>GHMGEVLTVFHAGSLSVPFEELEAEFEAQHPGVDVQREAAGSAQSVRKITELGKKADVLASADYALIPSLMVPEYADWYAAFARNQMILAYTNESKYGDEINTDNWYEILRRPDVRYGFSNPNDDPAGYRSQMVTQLAESYYNDDMIYDDLMLANTGMTLTTEENGTALIHVPASEEISPNTSKI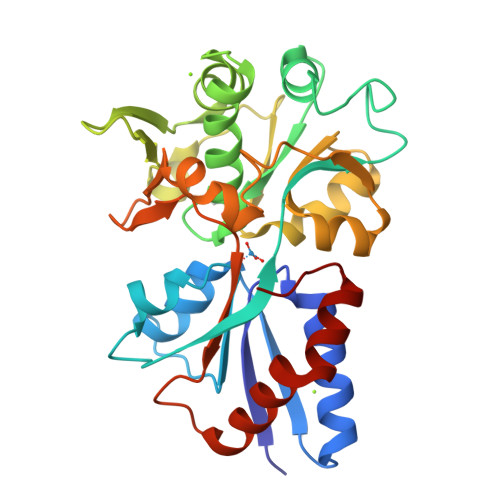MLRSMEVELSSALETGEIDYLYIYRSVAEQHGFEYVALPPAIDLSSLEYADNYSKVQVEMVNGEVVTGSPIVYGVTIPNNAENSELATEFVALLLGETGQQIFIENGQPPI[2x]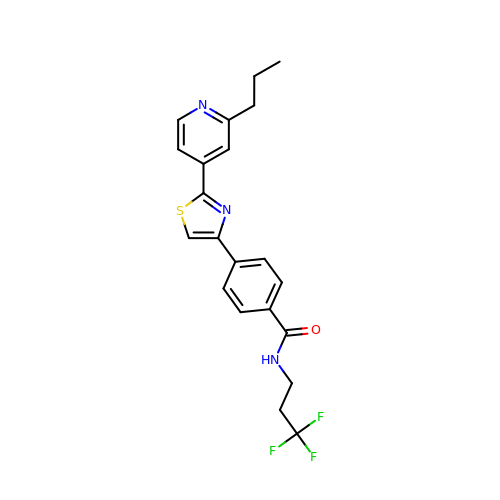4-[2-(2-propylpyridin-4-yl)-1,3-thiazol-4-yl]-~{N}-[3,3,3-tris(fluoranyl)propyl]benzamide | C21 H20 F3 N3 O S | QQMRZMWCFAMSQQ-UHFFFAOYSA-N>[2x]MLP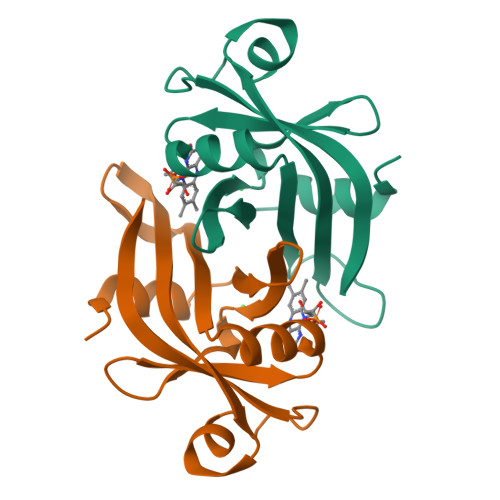GTFFEVLKNRGVVAIATQGEDGPHLVNTWNSYLKVLDGNRIVVPVGGMHKTEANVARDERVLMTLGSRKVAGRNGPGTGFLIRGSAAFRTDGPEFEAIARFKWARAALVITVVSAEQTL> MFKIVYPNAKDFFSFINSITNVTDSIILNFTEDGIFSRHLTEDKVLMAIMRIPKDVLSEYSIDSPTSVKLDVSSVKKILSKASSKKATIELTETDSGLKIIIRDEKSGAKSTI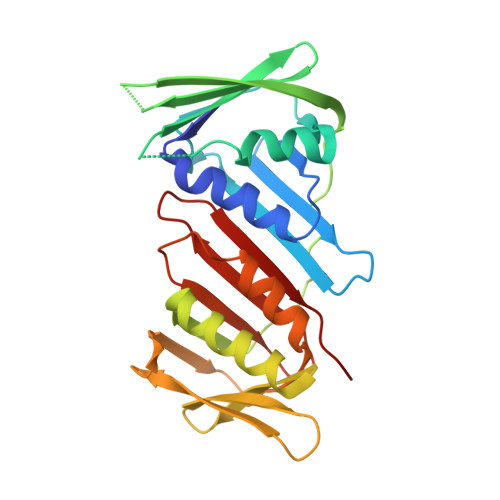YIKAEKGQVEQLTEPKVNLAVNFTTDESVLNVIAADVTLVGEEMRISTEEDKIKIEAGEEGKRYVAFLMKDKPLKELSIDTSASSSYSAEMFKDAVKGLRGFSAPTMVSFGENLPMKIDVEAVSGGHMIFWIAPRL>GPHMRKQEIIKTTEQLIEAVNNGDFE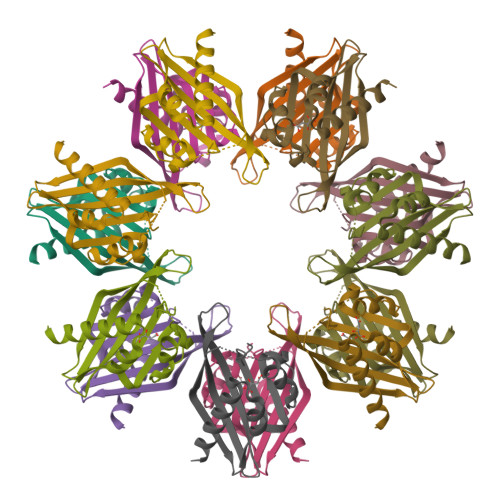AYAKICDPGLTSFEPEALGNLVEGMDFHRFYFENLLAKNSKPIHTTILNPHVHVIGEDAACIAYIRLTQYIDGQGRPRTSQSEETRVWHRRDGKWQNVHFHCSGAPVAPLQ[7x]>GSMSSQSQSPSVAQSIPSYLHADDLGPWGNYLQQVDRVAPYLGSLSRWIETLKRPKRILIVDVPIELDNGTVAHFEGYRVQHNVSRGPGKGGVRYHQDVTLSEVMALSAWMSVKNAAVNVPYGGAKGGIRVDPRKLSRGELERVTRRYTSEIGIIIGPNTDIPAPDVNT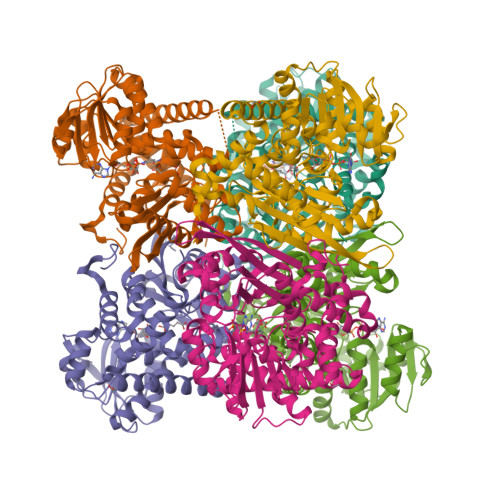NEQIMAWMMDTYSMNQGQTATGVVTGKPISLGGSLGRKEATGRGVFVVGCEAAKKKGVEIEGARIAVQGFGNVGGIAAKLFQEAGAKVIAVQDHTGTIHQPAGVDTAKLLDHVGRTGGVAGFEGAEPMPNDEFWTVETEILIPAALENQITEKNASKIRTKIIVEGANGPTTTAADDILSANGVLVIPDVIANAGGVTVSYFEWVQDFSSFFWTEDEINHRLERVMREAFAGVWAVAEEHKVSVRTAAFIVACKRILMAREMRGLYP[6x]>MGSSHHHHHHSQDPAGGNWTVFDEVLDSNVIKQLTLTGCGAACGEMLLRDRYIFVTQNVIGTELTSMTSLANKLNKFDVGWEGNAVSESSLYALSNTGSWGAMM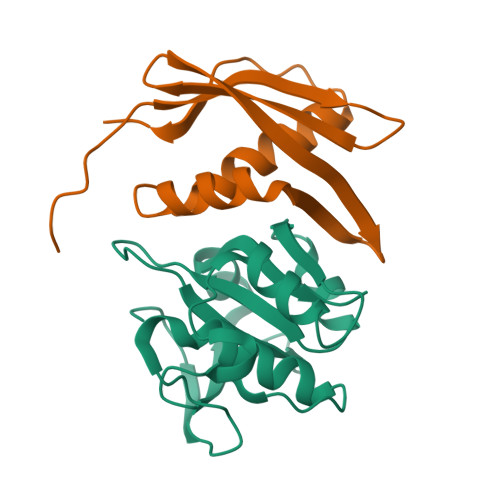WDSGSKVGHWVLVKGVDDAGNVIIYDPYQGSRYLMTEQEFKEVWNGHSVYKP[2x];>[2x]MGIVFTNHNIDLLSVEFDEITKNCNYTFSVDGETAIFTARISIIRNIKGIKYSEELDKFIMSIMPLQPKVSKILGGVTWDCICGKEVGFPVRLIGK Omapatrilat | C19 H24 N2 O4 S2 | 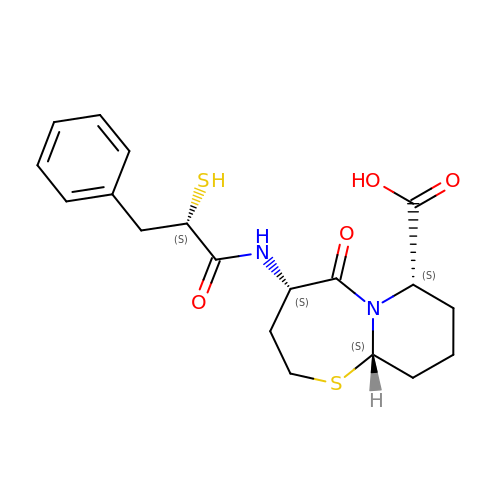LVRLSYPNFFBYCZ-VGWMRTNUSA-N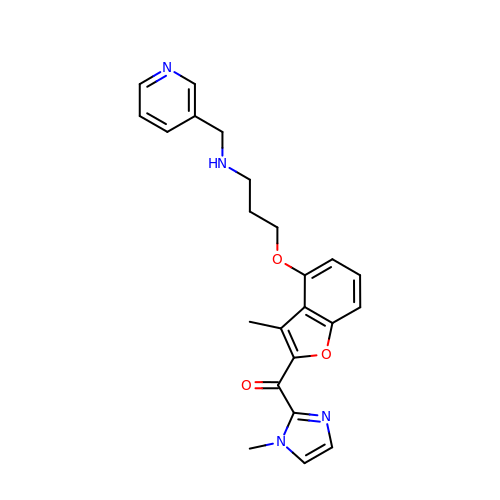(1-METHYL-1H-IMIDAZOL-2-YL)-(3-METHYL-4-{3-[(PYRIDIN-3-YLMETHYL)-AMINO]-PROPOXY}-BENZOFURAN-2-YL)-METHANONE | C23 H24 N4 O3 | VZBQJKIOAOUYJL-UHFFFAOYSA-N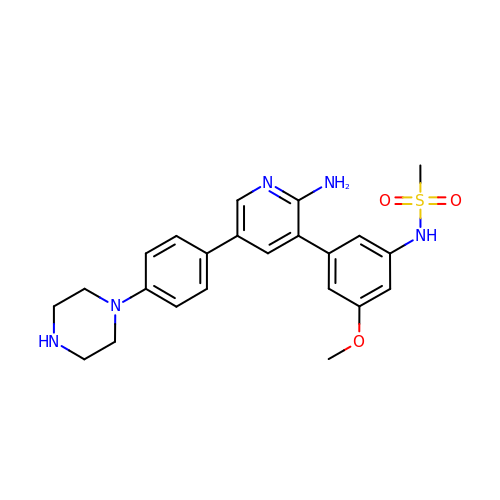~{N}-[3-[2-azanyl-5-(4-piperazin-1-ylphenyl)pyridin-3-yl]-5-methoxy-phenyl]methanesulfonamide | C23 H27 N5 O3 S | WTNLXMJMLHJDKF-UHFFFAOYSA-N> EVLFQGPKEDNIYNKLIKDDMTSGNYDNAQNIAKQTINKNYADDQTYYLSGMIMATINSKSEGMTEWERGLRMFPKSGLLNFELAIANRSLNDDE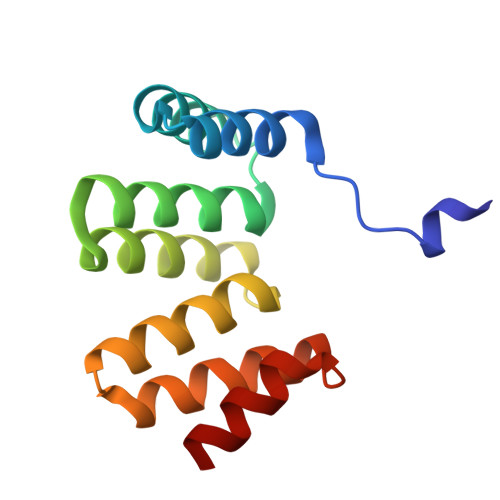KALKYVRKALNADPKNTDYINLEKELT>SDPSTGLPNKLFAFIGKTTASTSYVEKNLLSSTTGAAMVGLPSGGNLLQAQYFVTPEQFGAIGDGVTDDTQAILKTITFANTNNIQVRADKNYRFTSSIAMSGVRWYGGTFTGNGGTMISTVSCWMENVRFE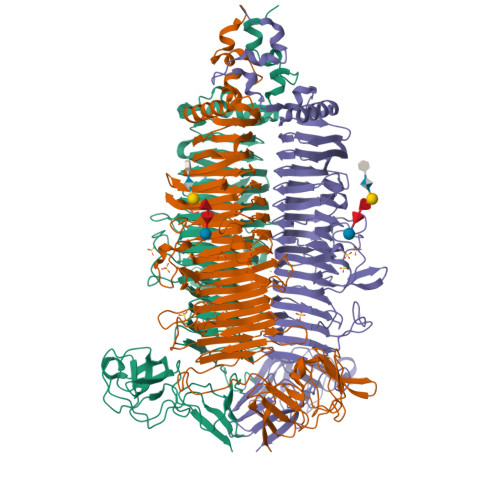KCYVKMLGGDCRFYRNIFSNATSTAAFLMQAMTSEGTLDFSYNEMYGCKYAILQQGTGEVMTYGRYSNNYIHDIKGDAIELNVVQKHYTEGLIIENNHIANVDASGQGANWGIGIGVAGSGPYGVDVPDSQYVRNFSIVGNRVYNCRQCLHVEMGKNFTIRDNEVYPNTAVSTGTGLTTCGVALYGCQDFEVDGLTGYLLNDPSVSTRMVFIDWGVNNGRYAGPPINFTIKNLDIPESSIEIATSGSDAWENSTIVSNINCNVFKWRGLPSSSTFNNIRCRSIDFIGQHGSGEGSGGGFYTRSQFTYMKWVGCTALSGDETTVSFAKIYTDRCDQVGNNFGVPTAVDGTGHRGPVLTTISEQYFTAYDEFPGGREFPTGTVIHCASGKKHVVTVGGAFFSDNEKIKATVTGQTYLQSNALNWASNGYAKAAGTKIVIPGAGANGGDLVTTIARATYVTNSLYTIDIADPIVTPTAENTQIKALNPVTFVTVNNA[2x]> MAAPLLDPLVSKLRQTTATAARAAEVMRAAFPGATHETAGRNTIAVQLPRKDVPTYVMANQRPQPWELLPMKAAAMTQYPNFFNNSCTFFGSIKRDVVNGVPFCLLRPSRLALDMAKVVRNLGIVDGFEVVQRRSRLGAHDFVWLPEQQPQEPEHLYDTSLFRQRLIRLHLRTDLFSRLPGAPGSGAGGPQPAS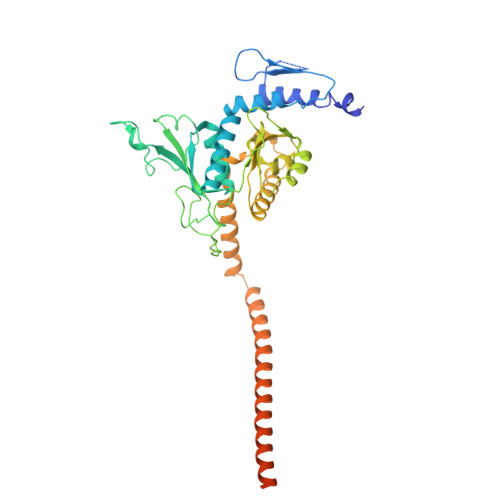AQLAPAVGLLPLSVKNISKASQPVLMYPRQLEEAAARLPAGVFMCYHPQLGLITDAMAQQYDVPALVAAHVGLPLSQAAAIRGALRVKAAEEAGKELRHVTQLKDWNMMELLRQRMVERRAALEAGMGVGGEVAARLQELREAGLRLRDEASDRVTSALNVAQDLEDGALAWQLVHSRALGAAPGAAAAGVDEGAGGEEQAGAGEGRTSPRGQPRRRR>MDWKKIYEDRTCTADEAVKSIKSGDRVLFAHCVAEPPVLVEAMVANAAAYKNVTVSHMVTLGKGEYSKPEYKENFTFEGWFTSPSTRGSIAEGHGQFVPVFFHEVPSLIRKDIFHVDVFMVMVSPPDHNGFCCVGVSSDYTMQAIKSAKIVLAEVNDQVPVVYGDTFVHVSEIDKFVETSHPLPEIGLPKIGEVEAAIGKHCASLIEDGSTLQLGIGAIPDAVLSQLKDKKHLGIHSEMISDGVVDLYEAGVIDCSQKSIDKGKMAITFLMGTKRLYDFAANNPKVELKPVDYINHPSVVAQCSKMVCINACLQVDFMGQIVSDSIGTKQFSGVGGQVDFVRGA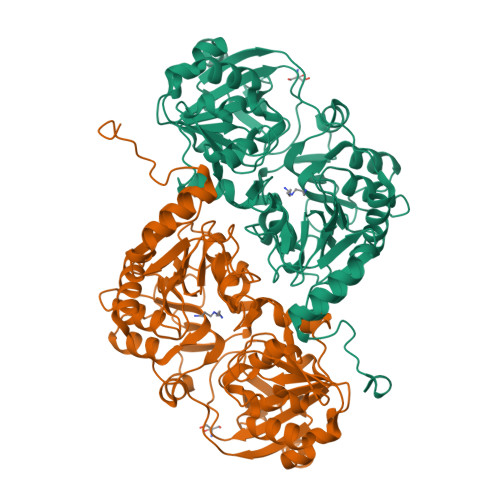SMSIDGKGKAIIAMPSVAKKKDGSMISKIVPFIDHGAAVTTSRNDADYVVTEYGIAEMKGKSLQDRARALINIAHPDFKDELKAEFEKRFNAAFSAWSHPQFEK[2x]> MLEQMISSSKVGVKINEWYKYIRLFSVPDSEIL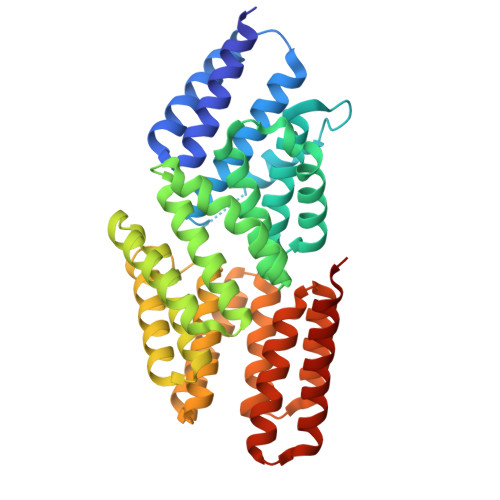KAEVEEEIRHMKEDHDLLLYYSLMCFRHQLMLDYLEPKTLNEERPKISDLLEKIESSQTDLKGILEYYFNFFRGMYEFEQYEYLNAISFYKQAERKLSLVADEIERAEFHYKVAEIYYHMKQTHMSMHHIVQAIDSYKAHENYTVRVIQCSFVIGLNYLDMDYPEKAIPHFKNALDKAREIDMSRLIGSSLYNLGLCSFAEEAYEKASEYFKEGIRVYQDNGYEHSNRILDILLMLTKTTFKMRNHSEGISWCAHGLSLSKNLNDEIMAKMFEFIHALYVDNDNEKLNSILNYLELKSMLSDVEDLASDAAKYYNEKEDHKVAVAYYEKVLYARKQIQRGDCLYET>[2x]GMSSMQHIVELTSDLIRFPSMHSRPEQISRCAGFIMDWCAQNGIHAERMDHDGIPSVMVLPEKGRAGLLLMAHIDVVDAEDDLFVPRVENDR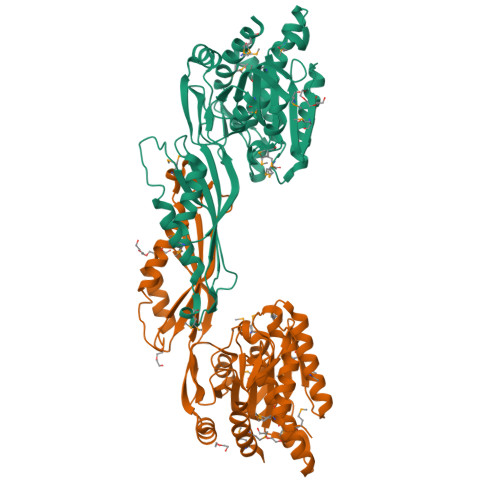LYGRGANDDKYAVALGLVMFRDRLNALKAAGRSQKDMALGLLITGDEEIGGMNGAAKALPLIRADYVVALDGGNPQQVITKEKGIIDIKLTCTGKAAHGARPWMGVNAVDLLMEDYTRLKTLFAEENEDHWHRTVNLGRIRAGESTNKVPDVAEGWFNIRVTEHDDPGALIDKIRKTVSGTVSIVRTVPVFLAADSPYTERLLALSGATAGKAHGASDARYLGENGLTGVVWGAEGFNTLHSRDECLHIPSLQSIYDPLMQLAREMEEHAAV>VPRGSAKGDGVTDDTAALTSALNDTPVGQKINGNGKTYKVTSLPDISRFINTRFVYERIPGQPLYYASEEFVQGELFKITDTPYYNAWPQDKAFVYENVIYAPYMGSDRAGVSRLHVSWVKSGDDGQTWSTPEWLTDLHPDYPTVNYHCMSMGVCRNRLFAMIETRTLAKNALTNCALWDRPMSRSLHLTGGITKAANQRYATIHVPDHGLFVGDFVNFSNSAVTGVSGDMTVATVIDKDNFTVLTPNQQTSDLNNAGKNWHMGTSFHKSPWRKTDLGLIPSVTEVHSFATIDNNGFAMGYHQGDVAPREVGLFYFPDAFNSPSNYVRRQIPSEYEPDASEPCIKYYDGVLYLITRGTRGDRLGSSLHRSRDIGQTWESLRFPHNVHHTTLPFAKVGDDLIMFGSERAENEWEAGAPD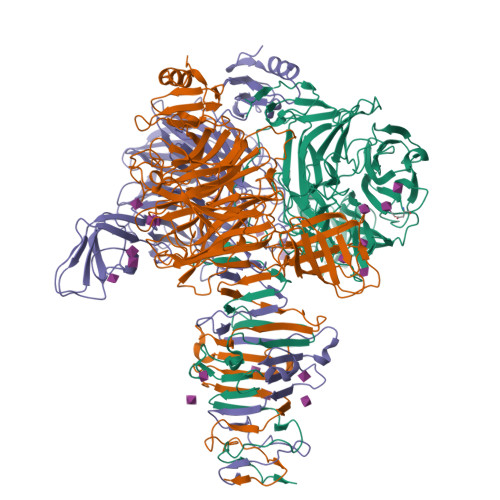DRYKASYPRTFYARLNVNNWNADDIEWVNITDQIYQGGIVNSGVGVGSVVVKDNYIYYMFGGEDHFNPWTYGDNSAKDPFKSDGHPSDLYCYKMKIGPDNRVSRDFRYGAVPNRAVPVFFDTNGVRTVPAPMEFTGDLGLGHVTIRASTSSNIRSEVLMEGEYGFIGKSIPTDNPAGQRIIFCGGEGTSSTTGAQITLYGANNTDSRRIVYNGDEHLFQSADVKPYNDNVTALGGPSNRFTTAYLGSNPIVT[3x]> GSMREYKLVVLGSVGVGKSALTVQFVQGIFVEKYDPTIEDSYRKQVEVDAQ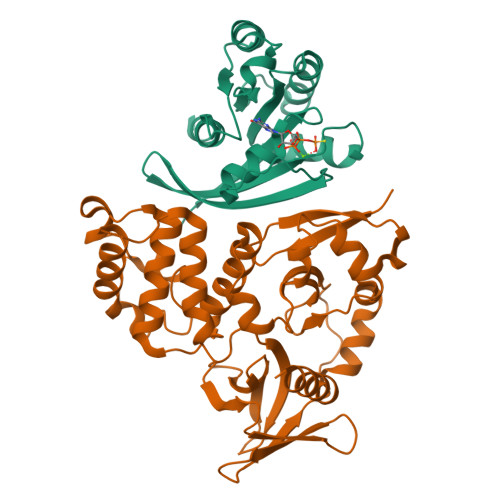QCMLEILDTAGTEQFTAMRDLYMKNGQGFALVYSITAQSTFNDLQDLREQILRVKDTDDVPMILVGNKCDLEDERVVGKEQGQNLARQWNNCAFLESSAKSKINVNEIFYDLVRQINR;> GSPEFEKVRIYRMDGSYRSVELKHGNNTTVQQIMEGMRLSQETQQYFTIWICSENLSLQLKPYHKPLQHVRDWPEILAELTNLDPQRETPQLFLRRDVRLPLEVEKQIEDPLAILILFDEARYNLLKGFYTAPDAKLITLASLLLQIVYGNYESKKHKQGFLNEENLKSIVPVTKLKSKAPHWTNRILHEYKNLSTSEGVSKEMHHLQRMFLQNCWEIPTYGAAFFTGQIFTKASPSNHKVIPVYVGVNIKGLHLLNMETKALLISLKYGCFMWQLGDTDTCFQIHSMENKMSFIVHTKQAGLVVKLLMKLNGQLMPTERNS> KPKYQVRWKIIESYEGNSYTFIDPTQLPYNEKWEFPRNNLQFGKTLGAGAFGKVVEATAFGLGKEDAVLKVAVKMLKSTAHADEKEALMSELKIMSHLGQHENIVNLLGACTHGGPVLVITEYCCYGDLLNFLRRKAEADLDKEDGRPLELRDLLHFSSQVAQGMAFLASKNCIHRDVAARNVLLTNGHVAKIGDFGLARDIMNDSNYIVKGNARLPVKWMAPESIFDCVYTVQSDVWSYGILLWEIFSLGLNPYPGILVNSKFYKLVKDGY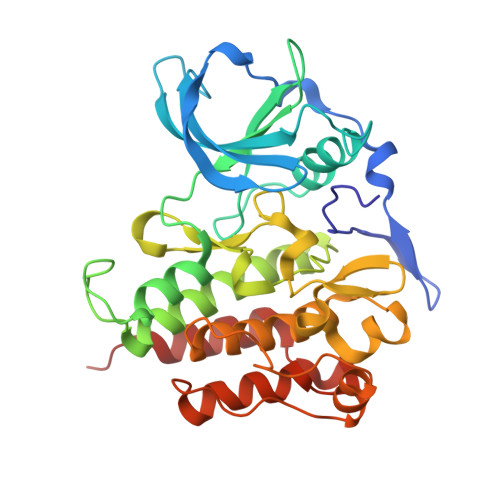QMAQPAFAPKNIYSIMQACWALEPTHRPTFQQICSFLQEQAQEDR> GSQQQEQPSTLAFILSQFNRDVYKWNFLDKVIDIMTTNFVSNTIRLLQPVPPFSLAGSKRKFETRTVVNIGEQLLLDLELLKEIFHTLPESVSNDSDLRENTSYKRVKRHADNNID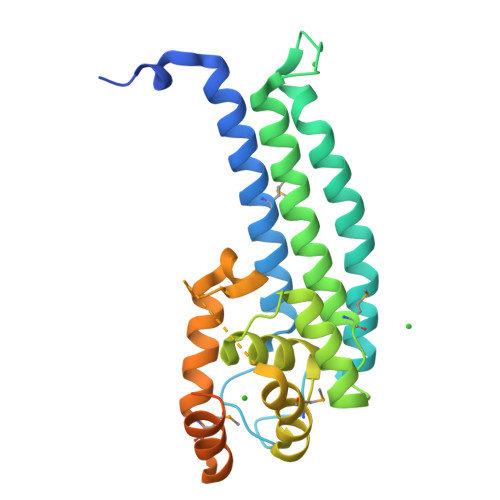QLLKFIKLLMAPLDSADDYYETYSKLTNNNPDSAVWSFVLALKGIPWDLALWKKMWSAYNLETDDTDEGSRPDSNRDLFIFKWDKVLLGQFENNLARMQDPNWSKFVRQDLKISPPVMKRIVSTPQIQQQKEEQKKQSLSVKDFVSHSRFFNRGT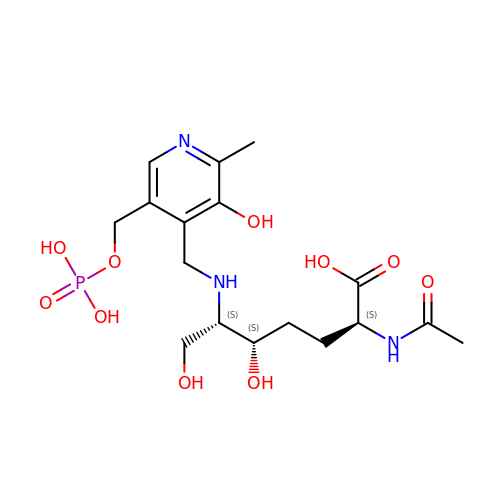(2~{S},5~{S},6~{S})-2-acetamido-6-[[2-methyl-3-oxidanyl-5-(phosphonooxymethyl)pyridin-4-yl]methylamino]-5,7-bis(oxidanyl)heptanoic acid | C17 H28 N3 O10 P | FNGADGGFBAIBRP-KKUMJFAQSA-N6-methylpyridine-2,3-dicarboxylic acid | C8 H7 N 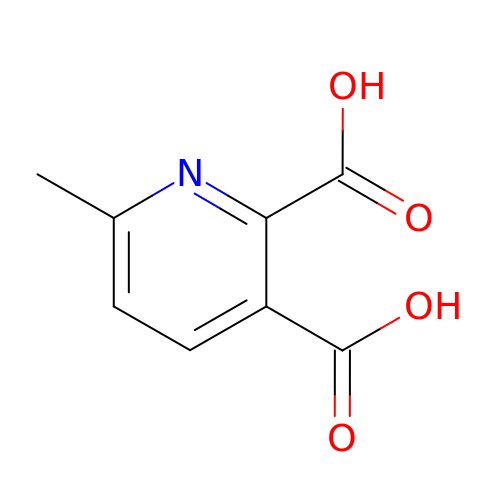O4 | PHQBKLKZIXCRIX-UHFFFAOYSA-N> TLSI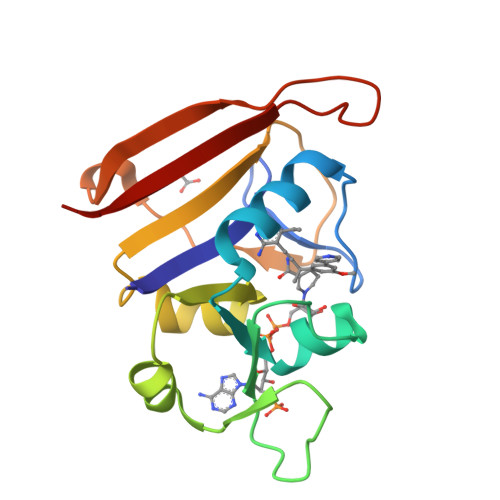LVAHDLQRVIGFENQLPWHLPNDLKHVKKLSTGHTLVMGRKTFESIGKPLPNRRNVVLTSDTSFNVEGVDVIHSIEDIYQLPGHVFIFGGQTLFEEMIDKVDDMYITVIEGKFRGDTFFPPYTFEDWEVASSVEGKLDEKNTIPHTFLHLIRK>GSASAKELACQEITVPLCKGIGYEYTYMPNQFNHDTQDEAGLEVHQFWPLVEIQCSPDLKFFLCSMYTPICLEDYKKPLPPCRSVCERAKAGCAPLMRQYGFAWPDRMRCDRLPEQGNPDTL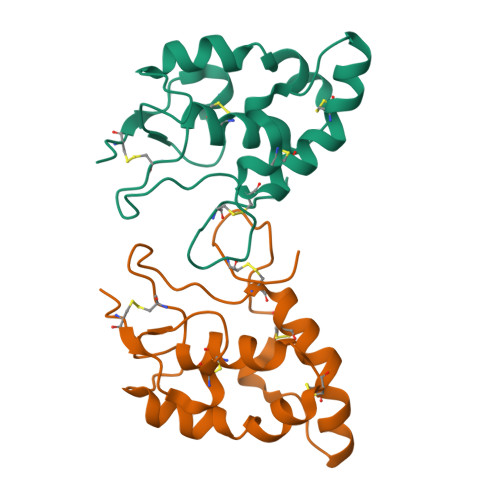CMDYERTD[2x]> MHHHHHHNNALGLV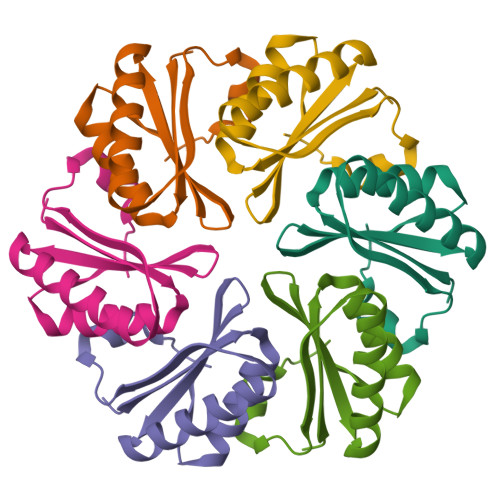ETKGLVGAIEAADAMVASANVQLVGYEKIGSGLVTVMVRGDVGAVKAAVDAGSAAASVVGEVKSCHVIPRPHSDVEAILPKSA>SPKLCLVCSDEASGCHYGVLTCGSCKVFFKRAVEGQHNYLCAGRNDCIIDKIRRKNCPACRYRKC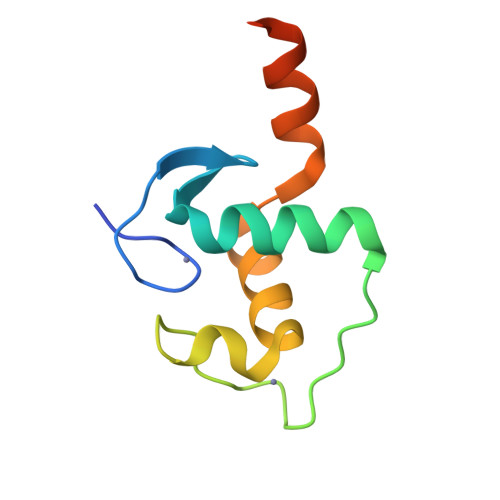LQAGMNLEARKTKKKIKGIQQATTG[8x]4-propan-2-ylphenol | C9 H12 O | 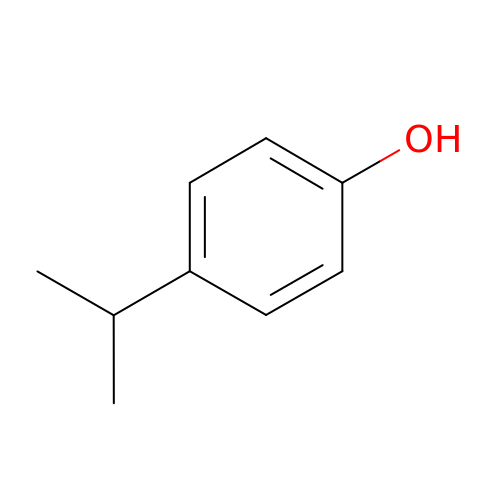YQUQWHNMBPIWGK-UHFFFAOYSA-N> MGSSHHHHHHSQGSTAPHHHVDDANSFVRAVERACSERGLRLTPIRANVLRLIADAGKPVKAYELLDWVREGKGVGADAP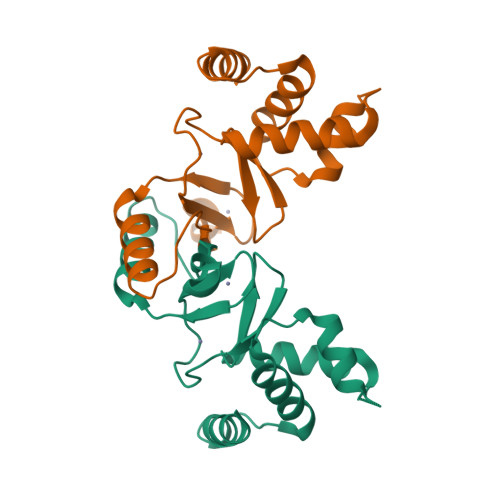PTVYRALDFLMANGFVHKLESVNAFVACHHPNSAQHSVPFLICDRCHSAVELEDRDVVSQLEARAKALGFQPQAQTLEVHGLCAKCAAAG>[2x]SSDTTPCCFAYIARPLPRAHIKEYFYTSGKCSN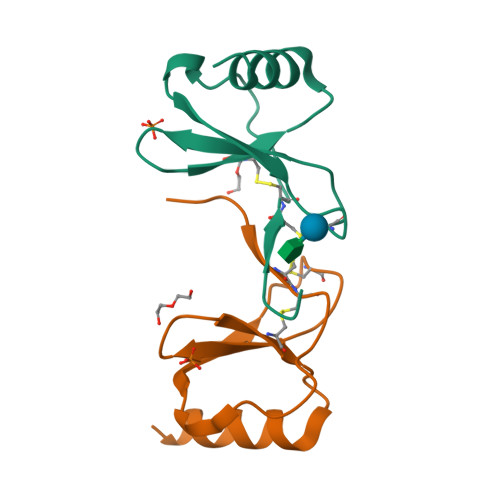PAVVFVTRKNRQVCANPEKKWVREYINSLEMS The interaction between NOT1 and CAF1/POP2 connects the NOT module to the catalytic module and thus is central to the assembly of the CCR4–NOT complex. Given the crucial role of this interaction, we have solved the crystal structures of the isolated CAF1-binding domain of human NOT1 (residues 1093–1317) at 2.90 Å resolution and its complex with CAF1 (i.e. CNOT7) at 2.70 Å resolution. The structures reveal that the CAF1-binding domain of NOT1 adopts an MIF4G fold; thus, this domain was termed the NOT1 MIF4G domain. CAF1 (i.e. CNOT7) and POP2 (i.e. CNOT8) are one-domain proteins that adopt an RNase D-like fold.

The structure of the isolated MIF4G domain of NOT1 was solved by molecular replacement using NOT1 coordinates from the NOT1–CAF1 complex as the search model. The crystallographic asymmetric unit contains six monomers that superimpose to the NOT1 chains in the complex with RMSDs of <0.7 Å, indicating that the NOT1 structure is not altered upon binding to CAF1. As predicted, the isolated MIF4G domain of NOT1 adopts a typical MIF4G fold composed of five HEAT-like antiparallel pairs of α-helices arranged into a right-handed solenoid. The HEAT-like repeats are followed by a C-terminal extension that wraps around α-helices α9 and α7 in a structurally conserved manner, independent of crystal contacts. Similarly the MIF4G domain of NOT1 does not undergo conformational changes upon binding to CAF1. A superposition of the NOT1 MIF4G domain with the third MIF4G domain of UPF2 yields an RMSD value of 2.8 Å, calculated from the positions of 190 alignable Cα atoms, despite a very low sequence identity (<8%). The most notable difference between the MIF4G domains of NOT1 and UPF2 is that the C-terminal extension of NOT1 is replaced by an additional helix (α-helix 11) in UPF2. Loop α3/α4 lies at the opposite side of the CAF1-binding site; the conservation of residues in this loop suggests that it may provide a binding site for an as-yet unidentified protein partner or other parts of NOT1.

>VLFQGPHMLEENIQEKIAFIFNNLSQSNMTQKVEELKETVKEEFMPWVSQYLVMKRVSIEPNFHSLYSNFLDTLKNPEFNKMVLNETYRNIKVLLTSDKAAANFSDRSLLKNLGHWLGMITLAKNKPILHTDLDVKSLLLEAYVKGQQELLYVVPFVAKVLESSIRSVVFRPPNPWTMAIMNVLAELHQEHDLKLNLKFEIEVLCKNLALDINELKPGNLLKDKDRLKNLDEQLS[6x]>[4x]MWFGEFGGQYVPETLIGPLKELEKAYKRFKDDEEFNRQLNYYLKTWAGRPTPLYYAKRLTEKIGGAKVYLKREDLVHGGAHKTNNAIGQALLAKFMGKTRLIAETGAGQHGVATAMAGALLGMKVDIYMGAEDVERQKMNVFRMKLLGANVIPVNSGSRTLKDAINEALRDWVATFEY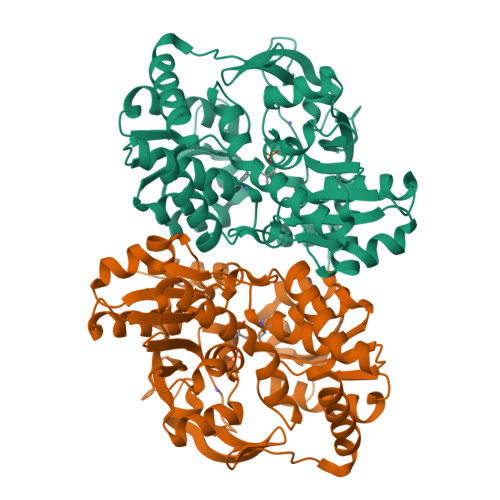THYLIGSVVGPHPYPTIVRDFQSVIGREAKAQILEAEGQLPDVIVACVGGGSNAMGIFYPFVNDKKVKLVGVEAGGKGLESGKHSASLNAGQVGVSHGMLSYFLQDEEGQIKPSHSIAPGLDYPGVGPEHAYLKKIQRAEYVAVTDEEALKAFHELSRTEGIIPALESAHAVAYAMKLAKEMSRDEIIIVNLSGRGDKDLDIVLKVSGNVLEHHHHHH> MGSSHHHHHHSSGPQQGLRQQEKPNFLIIQCDHLTQRVVGAYGQTQGCTLPIDEVASRGVIFSNAYVGCPLSQPSRAALWSGMMPHQTNVRSNSSEPVNTRLPENVPTLGSLFSESGYEAVHFGKTHDMGSLRGFKHKEPVAKPFTDPEFPVNNDSFLDVGTCEDAVAYLSNPPKEPFICIADFQNPHNICGFIGENAGVHTDRPISGPLPELPDNFDVEDWSNIPTPVQYICCSHRRMTQAAHWNEENYRHYIAAFQHYTKMVSKQVDSVLKALYSTPAGRNTIVVIMADHGDGMASHRMVTKHISFYDEMTNVPFIFAGPGIKQQKKPVDHLLTQPTLDLLPTLCDLAGIAVPAEKAGISLAPTLRGEKQKKSHPYVVSEWHSEYEYVTTPGRMVRGPRYKYTHYLEGNGEELYDMKK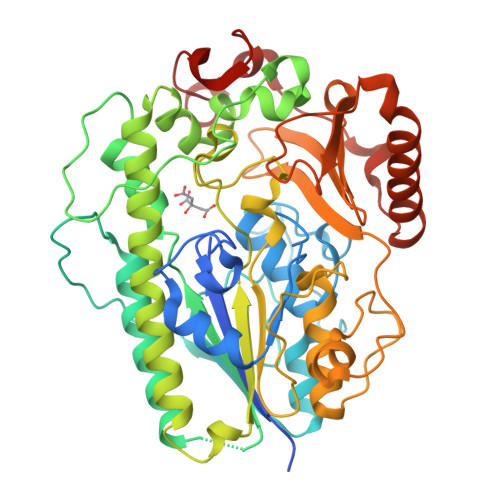DPGERKNLAKDPKYSKILAEHRALLDDYITRSKDDYRSLKVDADPRCRNHTPGYPSHEGPGAREILKRK~{N}-[3,3,3-tris(fluoranyl)propyl]benzenesulfonamide | C9 H10 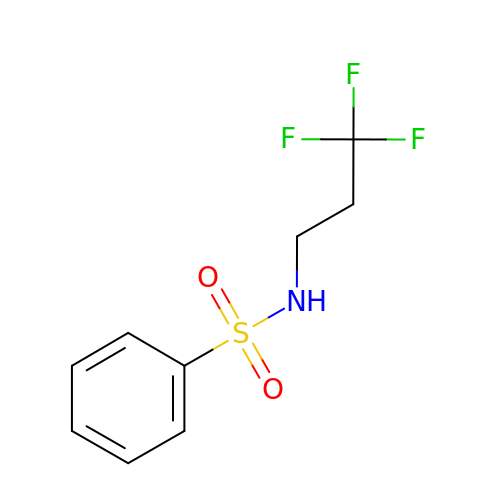F3 N O2 S | PCTNYPUVXBXHOS-UHFFFAOYSA-N(chloromethyl)benzene | C7 H7 Cl | 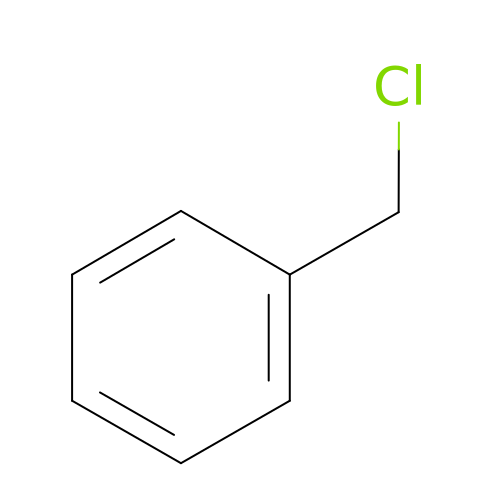KCXMKQUNVWSEMD-UHFFFAOYSA-N The AAA ATPase Vps4 drives the ESCRT (Endosomal Sorting Complexes Required for Transport) pathways that mediate membrane deformation and fission in a wide range of cellular processes. Vps4 is monomeric or dimeric in the cytosol, and assembles to form an active hexamer upon concentration at the membrane/ESCRT-III surface. The central pore of this hexamer is thought to be lined by pore loop 1 and pore loop 2 (residues 203–210 and 240–248, respectively), which are highly conserved in AAA ATPases that act on protein substrates and play a critical role in substrate translocation. The leading model is that the upstream factors recruit ESCRT-III subunits, which polymerize through their N-terminal domains to induce an inherently unstable membrane configuration that resolves by fission following Vps4-mediated disassembly or remodeling of the ESCRT-III polymer.

Guided by the insights that Vps4 is active as a hexamer that is stabilized by binding of ADP·BeFx and the VSL domain of the Vta1 cofactor, we used S. cerevisiae proteins to prepare a Vps4-Vta1VSL-ESCRT-IIIpeptide-ADP·BeFx complex for structural studies. Vps4 subunits A-D form a right-handed helix that is created by the three very similar interfaces formed by the A-B, B-C, and C-D subunit pairs. These interfaces each bury ~2000 Å2 of surface area and appear fashioned to coordinate ATP, with R288 and R289 from the neighboring Vps4 subunit positioned to coordinate the ATP phosphates. The D-E interface (~1700 Å2) is similar to the A-B, B-C, and C-D interfaces at the central pore region of the hexamer but deviates at the nucleotide-binding site, where the large AAA ATPase domain of subunit E is rotated by ~15° so that R288 and R289 are displaced by ~2 Å and are no longer able to coordinate see the nucleotide phosphates. The Vta1VSL dimers, which are pairs of helical hairpins that form a 4-helix bundle, stabilize the ring by forming struts between adjacent Vps4 subunits. Consistent with their more clearly defined density, the Vta1VSL dimers bound to the β domains of subunits A, B, C, and F also contact the small AAA ATPase domain of the following Vps4 subunit, with Y310’ and surrounding residues at the hairpin end of the second Vta1 subunit contacting α6 and α7 (residues 300–330) of the small AAA ATPase domain of the second Vps4. The primary contacts are with pore loop 1 (residues 203–209) of the A, B, C, and D Vps4 subunits, whose closest Cα atoms are ~7.5 Å from the helix axis that is defined by these loops. The peptide lies approximately along the helix axis, with Cα atoms modeled 1.0–2.7 Å (average 1.6 Å) from the axis, which is consistent with the model that substrates are translocated along or close to the helix axis, with some variation allowed to accommodate distinct amino acid sequences. Pore loop 1 of subunit F is displaced ~14 Å from the helix axis and is therefore completely disengaged from the substrate.

>MSTGDFLTKGIELVQKAIDLDTATQYEEAYTAYYNGLDYLMLALKYEKNPKSKDLIRAKFTEYLNRAEQLKKHLESEEANAAKKSPSAGSGSNGGNKKISQEEGEDNGGEDNKKLRGALSSAILSEKPNVKWEDVAGLEGAKEALKEAVILPVKFPHLFKGNRKPTSGILLYGPPGTGKSYLAKAVATEANSTFFSVSSSDLVSKWMGESEKLVKQLFAMARENKPSIIFIDEVDALTGTRGEGESEASRRIKTELLVQMNGVGNDSQGVLVLGATNIPWQLDSAIRRRFERRIYIPLPDLAARTTMFEINVGDTPCVLTKEDYRTLGAMTEGYSGSDIAVVVKDALMQPIRKIQSATHFKDVSTEDDETRKLTPCSPGDDGAIEMSWTDIEADELKEPDLTIKDFLKAIKSTRPTVNEDDLLKQEQFTRDFGQEGN[6x];>[12x]MASNAARVVATAKDFDKVGLGIIGYYLQLYAVELILSEEDRSQEMTALATELLDTIEAFKKEIGGESEAEDSDKSLHVMNTLIHDQEKAKIYMLNFTMSLYNEKLKQLKDGPWDVMLKRSLWCCIDLFSCILHLWKENISETSTNSLQKRIKYCKIYLSKLAKGEIGSSDEKTLDYADFADDSEEIKDEDVDHQTSDLENNNNDKVEGLAPKDQTTSYEPVDEVPEFIDDADSVNEEEQTVDKNEDAITKDEQQVVKKEVDLTRPSAPSEPAAAEHKSYTKDELTKIMDRASKIEQIQKLAKYAISALNYEDLPTAKDELTKALDLLNSI(2S,3S)-3-FORMYL-2-({[(4-METHYLPHENYL)SULFONYL]AMINO}METHYL)PENTANOIC 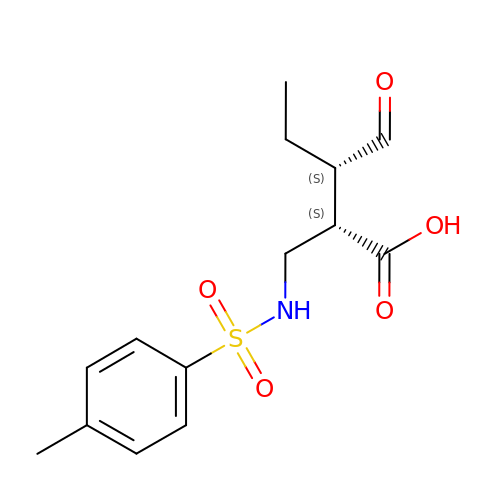ACID | C14 H19 N O5 S | IDDWUPNJUMHKFQ-DGCLKSJQSA-N>MVIKAQSPAGFAEEYIIESIWNNRFPPGTILPAERELSELIGVTRTTLREVLQRLARDGWLTIQHGKPTKVNNFWETSGLNILETLARLDHESVPQLIDNLLSVRTNISTIFIRTAFRQHPDKAQEVLATANEVADHADAFAELDYNIFRGLAFASGNPIYGLILNGMKGLYTRIGRHYFANPEARSLALGFYHKLSALCSEGAHDQVYETVRRYGHESGEIWHRM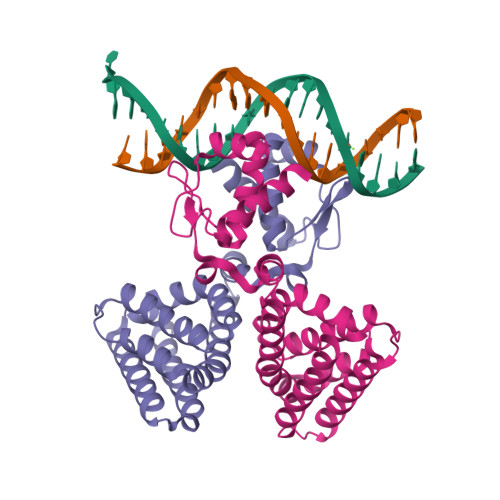QKNLPGDLAIQGR[2x]>HHHHHHENLYFQGMSFDNYLVPTVIEQSGRGE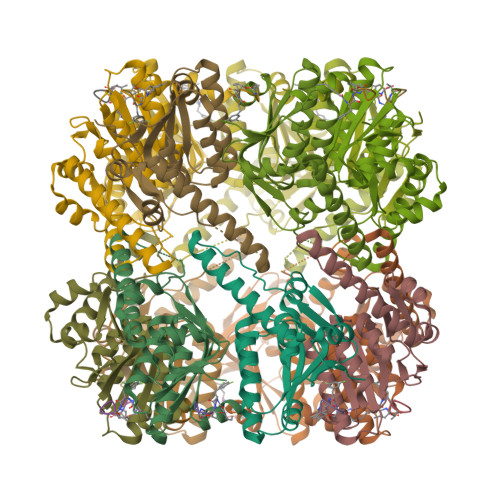RAFDIYSRLLKERIVFLVGPVTDESANLVVAQLLFLESENPDKDIFFYINSPGGSVTAGMSIYDTMNFIKPDVSTLCLGQAASMGAFLLSAGEKGKRFALPNSRIMIHQPLISGGLGGQASDIEIHARELLKIKEKLNRLMAKHCDRDLADLERDTDRDNFMSAEEAKEYGLIDQILENRASLRL[28x]> MDWSHPQFEKKKKAEWPRKLRSQEWYGGTSRDVIYHRGWLKNQGYPHDLFDGRPVIGILNTWSDMTPCNGHLRELAEKVKAGVWEAGGFPLEVPVFSASENTFRPTAMMYRNLAALAVEEAIRGQPMDGCVLLVGCDKTTPSLLMGAASCDLPSIVVTGGPMLNGYFRGERVGSGTHLWKFSEMVKAGEMTQAEFLEAEASMSRSSGTCNTMGTASTMASMAEALGMALSGNAAIPGVDSRRKVMAQLTGRRIVQMVKDDLKPSEIMTKQAFENAIRTNAAIGGSTNAVIHLLAIAGRVGIDLSLDDWDRCGRDVPTIVNLMPSGKYLMEEFFYAGGLPVVLKRLGEAGLLHKDALTVSGETVWDEVKDVVNWNEDVILPAEKALTSSGGIVVLRGNLAPKGAVLKPSAASPHLLVHKGRAVVFEDIDDYKAKINDDNLDIDENCIMVMKNCGPKGYPGMAEVGNM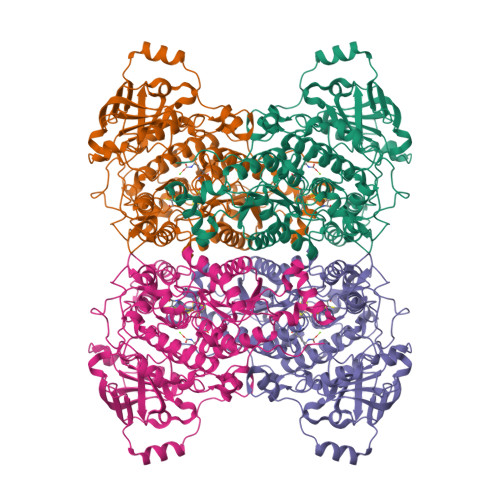GLPPKVLKKGILDMVRISDARMAGTAYGTVVLHTSPEAAVGGPLAVVKNGDMIELDVPNRRLHLDISDEELARRLAEWQPNHDLPTSGYAFLHQQHVEGADTGADLDFLKGCRGNAVGKDSH>[2x]MQEQRQQLLRSLEALIFSSEEPVNLQTLSQITAHKFTPSELQEAVDELNRDYEATGRTFRIH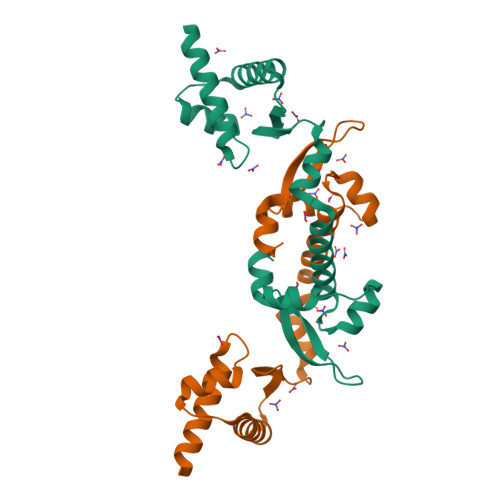AIAGGYRFLTEPEFADLVRQLLAPVIQRRLSRSMLEVLAVVAWHQPVTKGEIQQIRGASPDYSIDRLLARGLIEVRGRADSPGRPLQYGTTEVFLDLFHL N-ethyl-3-(1-methyl-1H-1,2,3-triazol-4-yl)-4-(pyridin-2-ylmethoxy)benzamide 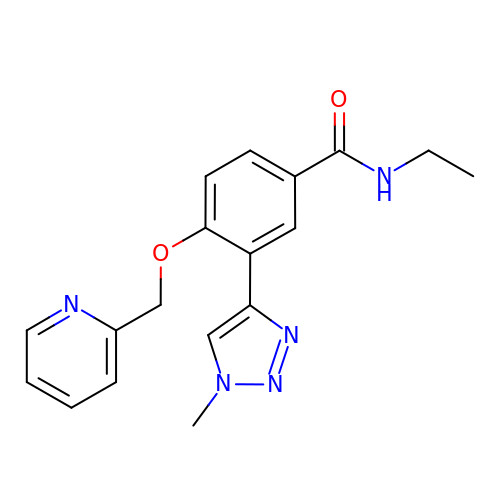| C18 H19 N5 O2 | PXCVJESJJFPBNT-UHFFFAOYSA-N>MNANLFARLFDKLDDPHKLAIETAAGDKISYAELVARAGRVANVLVARGLQVGDRVAAQTEKSVEALVLYLATVRAGGVYLPLNTAYTLHELDYFITDAEPKIVVCDPSKRDGIAAIAAKVGATVETLGPDGRGSLTDAAAGASEAFATIDRGADDLAAILYTSGTTGRSKGAMLSHDNLASNSLTLVDYWRFTPDDVLIHALPIYHTHGLFVASNVTLFARGSMIFLPKFDPDKILDLMARATVLMGVPTFYTRLLQSPRLTKETTGHMRLFISGSAPLLADTHREWSAKTGHAVLERYGMTETNMNTSNPYDGDRVPGAVGPALPGVSARVTDPETGKELPRGDIGMIEVKGPNVFKGYWRMPEKTKSEFRDDGFFITGDLGKIDERGYVHILGRGKDLVITGGFNVYPKEIESEIDAMPGVVESAVI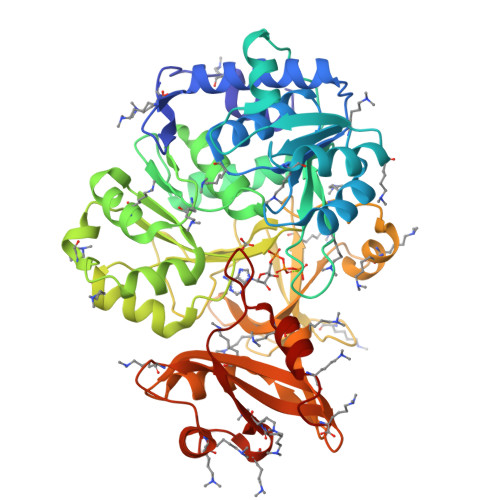GVPHADFGEGVTAFVVLKREFAPSEILAEELKAFVKDRLAKFKMPKKVIFVDDLPRNTMGAVQKNVLRETYKDIYK[3x]>[2x]MSALFEPYTLKDVTLRNRIAIPPMCQFMAEDGLINDWHQVHYASMARGGAGLLVVEATAVAPEGRITPGCAGIWSDAHAQAFVPVVQAIKAAGSVPGIQIAHAGRKASANRPWEGDDHIGADDARGWETIAPSAIAFGAHLPNVPRAMTLDDIARVKQDFVDAARRARDAGFEWIELHFAHGYLGQSFFSEHSNKRTDAYGGSFDNRSRFLLETLAAVREVWPENLPLTARFGVL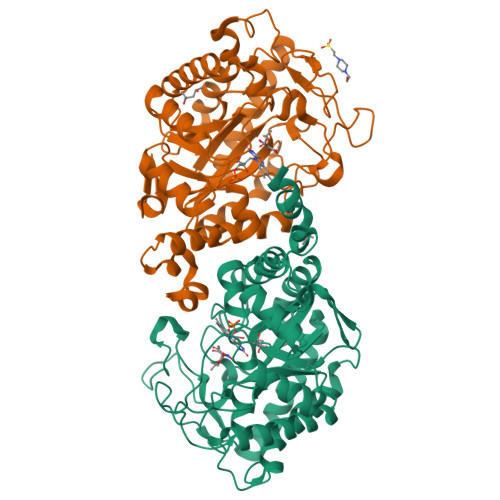EYDGRDEQTLEESIELARRFKAGGLDLLSVSVGFTIPETNIPWGPAFMGPIAERVRREAKLPVTSAWGFGTPQLAEAALQANQLDLVSVGRAHLADPHWAYFAAKELGVEKASWTLPAPYAHWLERYRLEHHHHHH>AGGLVPMVVEQSARGERAYDIYSRLLKERIIFLVGQVEDYMANLVVAQLLFLEAENPEKDIHLYINSPGGSVTAGMSIYDTMQFIKPNVSTTCIGQACSMGALLLAGGAAGKRYCLPHSRMMIHQPLGGFQGQASDIEIHAKEILFIKERLNQILAHHTGQPLDVIARDTDRDRFMSGDEAVKYGLIDKVMTQRDL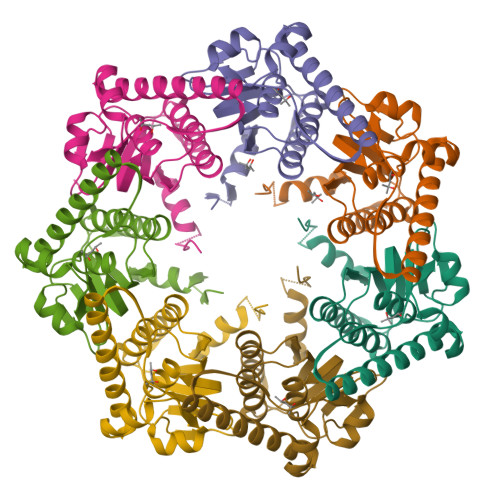AVSGSGSGHHHHHH[14x]> GDSIEDKNARVIELIAAYRNRGHLMADIDPLRLDNTRFRSHPDLDVNSHGLTLWDLDREFKVDGFAGVQRKKLRDILSVLRDAYCRHVGVEYTHILEPEQQRWIQERVETKHDKPTVAEQKYILSKLNAAEAFETFLQTKYVGQKRFSLEGAETVIPMMDAVIDQCAEHGLDEVVIAMPHRGRLNVLANIVGKPYSQIFSEFEGNLNPSQAHGSGDVKYHLGATGTYIQMFGDNDIEVSLTANPSHLEAVDPVL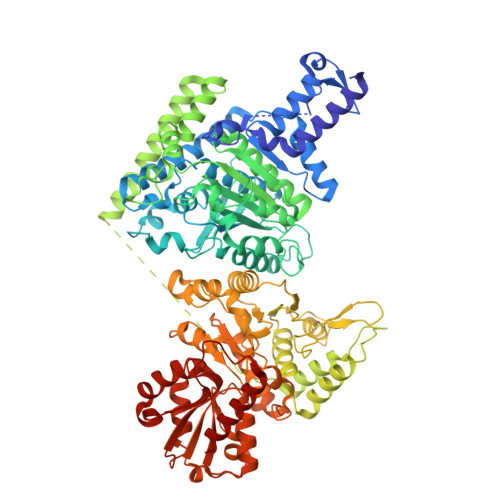EGLVRAKQDLLDTGEEGSDNRFSVVPLMLHGDAAFAGQGVVAETLNLALLRGYRTGGTIHIVVNNQIGFTTAPTDSRSSEYCTDVAKMIGAPIFHVNGDDPEACAWVARLAVDFRQAFKKDVVIDMLCYRRRGHNEGDDPSMTQPYMYDVIDTKRGSRKAYTEALIGRGDISMKEAEDALRDYQGQLERVFNEVRELEKHEIEPSESVEADQQIPSKLATAVDKAMLQRIGDAHLALPEGFTVHPRVRPVLEKRREMAYEGRIDWAFAELLALGSLIAEGKLVRLSGQDTQRGTFTQRHAVIVDRKTGEEFTPLQLLATNPDGTPTGGKFLVYNSALSEFAAVGFEYGYSVGNPDAMVLWEAQFGDFVNGAQSIIDEFISSGEAKWGQLSDVVLLLPHGHEGQGPDHTSGRIERFLQLWAEGSMTIAMPSTPANYFHLLRRHGKDGIQRPLIVFTPKSMLRNKAAVSDIRDFTESKFRSVLEEPMYTDGEGDRNKVTRLLLTSGKIYYELAARKAKENREDVAIVRIEQLAPLPRRRLAETLDRYPNVKEKFWVQEEPANQGAWPSFGLTLPEILPDHFTGLKRISRRAMSAPSSGSSKVHAVEQQEILDTAFG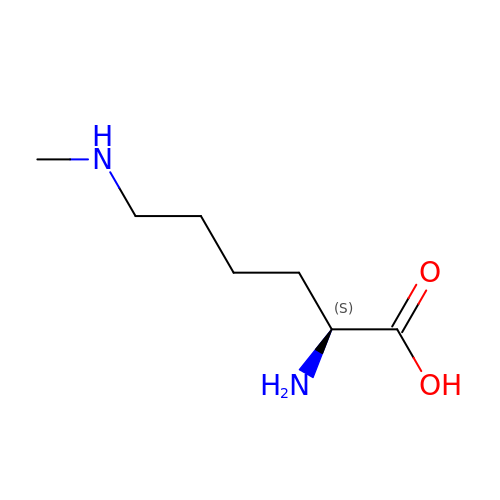N-METHYL-LYSINE | C7 H16 N2 O2 | PQNASZJZHFPQLE-LURJTMIESA-N> MPNTAMKKKVLLMGKSGSGKTSMRSIIFANYIARDTRRLGATIDVEHSHVRFLGNLVLNLWDCGGLDTFMENYFTSQRDNIFRNVEVLIYVFDVESRELEKDMHYYQSCLEAILQNSPDAKIFCLVHKMDLVQEDQRDLIFKEREEDLRRLSRPLECACFRTSIWDETLYKAWSSIVYQLIPNVQQLEMNLRNFAQIIEADEVLLFERATFLVISHYQCKEQRDVHRFEKISNIIKQFKLSCSKLAASFQSMEVRNSNFAAFIDIFTSNTYVMVVMSDPSIP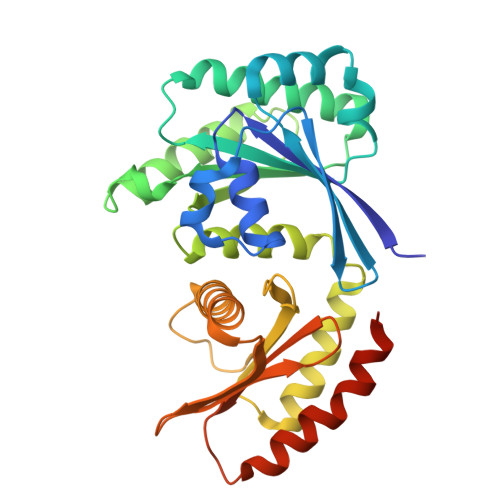SAATLINIRNARKHFEKLERVDGPKHSLLMR> ATHTAQTQT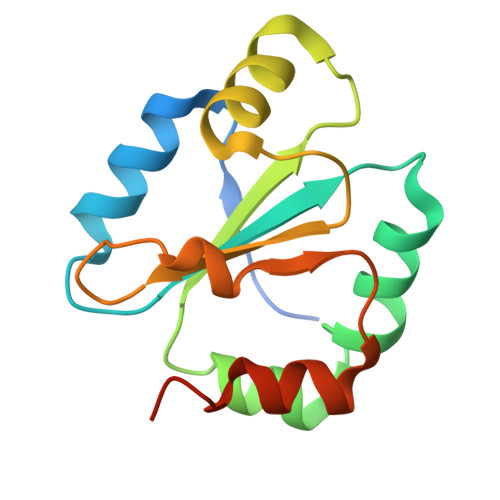HLNFTQIKTVDELNQALVEAKGKPVMLDLYADWCVASKEFEKYTFSDPQVQKALADTVLLQANVTANDAQDVALLKHLNVLGLPTILFFDGQGQEHPQARVTGFMDAETFSAHLRDRQPHHHHHH> ANLRLSEANSGTYKTFIG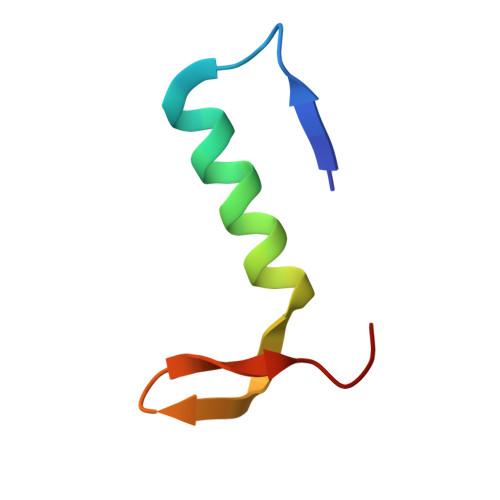RVREELGSETYRLYGIPVLKHSL> XYC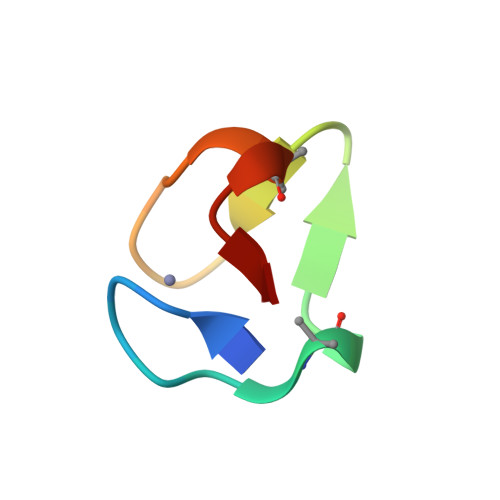SDCGADASQVRGGYCTNCGASADRIRX> PSFDCGKPQVEPKKCPGRVVGGCVAHPHSWPWQVSLRTRFGMHFCGGTLISPEWVLTAAHCLEKSPRPSSYKVILGAHQEVNLEPHVQEIEVSRLFLEPTRKDIALLKLSSPAVITDKVIPACLPSPNYVVADRTECFITGWG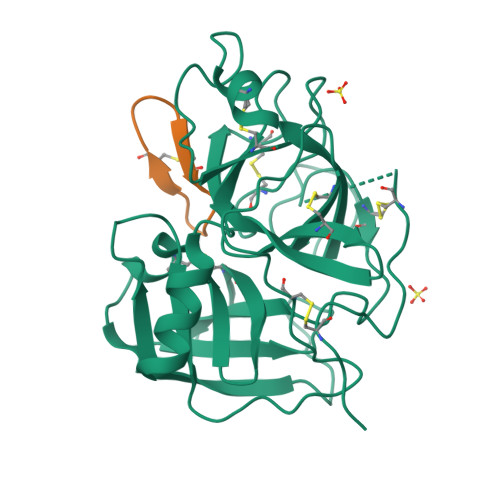ETQGTFGAGLLKEAQLPVIENKVCNRYEFLNGRVQSTELCAGHLAGGTDSCQGDSGGPLVCFEKDKYILQGVTSWGLGCARPNKPGVYVRVSRFVTWIEGVMRNN;> GRCYKSIPPICFPD>TLKLCSPEEFTRLCREKTQEIYPIKEANGRTRKALIICNTEFKHLSLRYGANFDIIGMKGLLEDLGYDVVVKEELTAEGMESEMKDFAALSEHQTSDS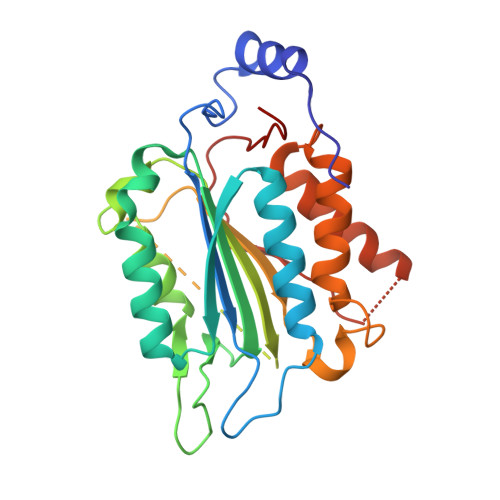TFLVLMSHGTLHGICGTMHSEKTPDVLQYDTIYQIFNNCHCPGLRDKPKVIIVQAARGGNSGEMWIRESSKPQLCRGVDLPRNMEADAVKLSHVEKDFIAFYSTTPHHLSYRDKTGGSYFITRLISCFRKHACSCHLFDIFLKVQQSFEKASIHSQMPTIDRATLTRYFYLFPGN[4x]> QNGYV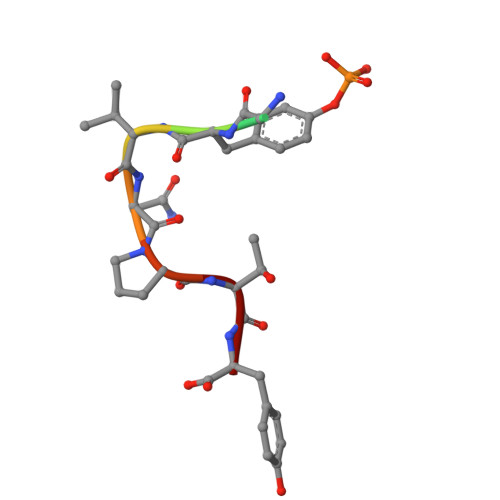NPTY> MSSNNSGLSAAGEIDESLYSRQLYVLGKEAMLKMQTSNVLILGLKGLGVEIAKNVVLAGVKSMTVFDPEPVQLADLSTQFFLTEKDIGQKRGDVTRAKLAELNAYVPVNVLDSLDDVTQLSQFQVVVATDTVSLEDKVKINEFCHSSGIRFISSETRGLFGNTFVDLGDEFTVLDPTGEEPRTGMVSDIEPDGTVTMLDDNRHGLEDGNFVRFSEVEGLDKLNDGTLFKVEVLGPFAFRIGSVKEYGEYKKGGIFTEVKVPRKISFKSLKQQLSNPEFVFSDFAKFDRAAQLHLGFQALHQFAVRHNGELPRTMNDEDANELIKLVTDLSVQQPEVLGEGVDVNEDLIKELSYQARGDIPGVVAFFGGLVAQEVLKACSGKFTPLKQFMYFDSLESLPDPKNFPRNEKTTQPVNSRYDNQIAVFGLDFQKKIANSKVFLVGSGAIGCEMLKNWALLGLGSGSDGYIVVTDNDSIEKSNLNRQFLFRPKDVGKNKSEVAAEAVCAMNPDLKGKINAKIDKVGPETEEIFNDSFWESLDFVTNALDNVDARTYVDRRCVFYRKPLLESGTLGTKGNTQVIIPRLTESYSSSRDPPEKSIPLCTLRSFPNKIDHTIAWAKSLFQGYFTDSAENVNMYLTQPNFVEQTLKQSGDVKGVLESISDSLSSKPHNFEDCIKWARLEFEKKFNHDIKQLLFNFPKDAKTSNGEPFWSGAKRAPTPLEFDIYNNDHFHFVVAGASLRAYNYGIKSDDSNSKPNVDEYKSVIDHMIIPEFTPNANLKIQVNDDDPDPNANAANGSDEIDQLVSSLPDPSTLAGFKLEPVDFEKDDDTNHHIEFITACSNCRAQNYFIETADRQKTKFIAGRIIPAIATTTSLVTGLVNLELYKLIDNKTDIEQYKNGFVNLALPFFGFSEPIASPKGEYNNKKYDKIWDRFDIKGDIKLSDLIEHFEKDEGLEITMLSYGVSLLYASFFPPKKLKERLNLPITQLVKLVTKKDIPAHVSTMILEICADDKEGEDVEVPFITIHL

The covalent modification of target proteins with ubiquitin or ubiquitin-like modifiers is initiated by E1 activating enzymes, which typically transfer a single modifier onto cognate conjugating enzymes. UBA6 is an unusual E1 since it activates two highly distinct modifiers, ubiquitin and FAT10. In the presence of Mg-ATP, E1 catalyzes the acyl-adenylation of ubiquitin, initially forming a ubiquitin-AMP adduct. Subsequently, the E1 catalytic cysteine attacks the ubiquitin-AMP intermediate to form a thioester bond between the cysteine and the C-terminal glycine of ubiquitin, resulting in the formation of a covalent E1~ubiquitin adduct.

As the resolution of the UBA6-ATP complex did not permit a detailed analysis of the interactions between Mg2+-ATP and the protein, in particular the coordination of the two metal cations, which could be visualized in the maps, we determined the structure of yeast Uba1 in complex with Mg2+-ATP at high resolution. These crystals diffracted X-rays also anisotropically, and, after processing with Staraniso, resolutions of 1.72 Å in the best direction and 2.24 Å in the weakest direction were obtained. Refinement resulted in a high-quality model in which the majority of residues, including the bound ATP together with bound metal ions and the surrounding residues, were well defined. Somewhat surprisingly, two octahedrally coordinated magnesium ions instead of one were observed to interact with the triphosphate moiety of the nucleotide. The first Mg-ion, Mg(1), is coordinated by the side chain of D544, one oxygen each of the α, β and γ phosphates and two water molecules, while Mg(2) interacts with the side chain of D472, one oxygen of the β phosphate and four water molecules. The triphosphate moiety is also recognized by R21 from the IAD and R481 from the AAD which interact with the γ phosphate and the oxygen atom bridging the β and γ phosphate. Finally, K494 contacts the bridging oxygen between the α and β phosphate and the 3’ OH-group. The 2’ and 3’ OH-groups of the ribose engage in H-bonds with the carboxylate of D470, while the base interacts with the side chain amide of N545 and both main chain atoms of V520. Comparing the contribution of the two acidic residues revealed that only D544 is critical for ATP hydrolysis since the D544A variant was almost completely impaired. In the Uba1-ATP complex the side chain of R590 points, to a first approximation, towards the bound ATP while it is reoriented away from the nucleotide binding site in both ubiquitin-bound structures.In Gram-positive pathogens such as Staphylococcus aureus (Sa) and Enterococcus faecalis (Ef), the pleiotropic transcription factor CodY plays a key role in integrating metabolism and virulence factor expression. CodY DNA-binding is activated by two types of ligands: branched chain amino acids (BCAAs, i.e. isoleucine, leucine, and valine) and, in most cases, guanosine triphosphate, GTP. Each 30 kDa protomer comprises the N-terminal ligand-binding domain called GAF (cGMP-specific phosphodiesterases, adenylyl cyclases and FhlA). The GAF domain is connected by an extended linker helix to the C-terminal DNA-binding (DBD) domain that contains a winged helix-turn-helix (wHTH) motif.

Fortunately, the crystal structure of the EfCodY-DNA complex—presented in more detail below—had Leu-bound GAF domains. The EfCodY complex was co-crystallized in the presence of Leu, yet Leu bound only to protomers A and B (dimer 1). In protomers C and D (dimer 2), the residues Glu58-Lys75 involved in the H3-helix shift had overall weaker electron density compared to ligand-free EfCodY. In the crystals, two CodY dimers bind to a single DNA duplex. In the Ef-complex, the DBD domains of the two dimers are related by a 60° rotation as in the Sa-complex; however, their GAF domains are related by a ∼45° rotation due to a shift in the position of the N-terminal parts of the linker helices. Leu binding induces the H3-formation associated with a large displacement of loop residues Lys74, Lys75 and Phe76. These residues now reside in the H3-H4 linker forming a ß-sheet interaction with Gly51, Asp52 and Leu53 in the S1–S2 loop—similar to what we observed in SaCodY. Arg66 moved into the position of Lys74 and occupies the equivalent position to Arg61 in Ile/GTP-activated SaCodY, forming a salt bridge with the carboxylate group of the bound Leu-molecule. Importantly, Lys74 in the H3–H4 linker, stabilized by the ß-sheet, now moved close enough to the H1–H2 loop to form a direct salt bridge with the insertion residue Glu26. In EfCodY, the structural changes in the BCAA-binding site are thus directly coupled to changes in the H1–H2 loop—as opposed to via GTP in SaCodY.

>[4x]GAMATLLEKTRQVNELLQKNNLFDVQAELPYNKMAMILGDILESNAYIISSSGDLLGYTEKLDVNNARIKNMFKEKKFPQGYTEAVDMLKVTEANIPIDSDLTAFPFESRELYPFGLTTIVPLYGAGKRLGTIILARVEKSFNEDDLVLAEYSATVVGMQILYHQSRTIEAEVRSATAVQMAINTLSYSELKAVHAIFEALDGEEGRLTASSIADEIGITRSVIVNALRKLESAGIIESRSLGMKGTYLKVLNQQFIKELEK GQs consist of four-stranded nucleic acid helical structures formed by the stacking of two or more guanine tetrads and stabilised by monovalent cations. GQ motifs are in fact over-represented at the ends of chromosomes, in telomeres, being involved in maintaining chromosome stability. GQ motifs are often able to inhibit telomerase action and obstruct DNA replication and repair, leading to activation of the DNA damage response pathway that results in apoptosis. The ligands reported feature a berberine G-quadruplex stabiliser scaffold connected to a moiety inhibiting hCAs IX and XII.

Crystals suitable for X-ray diffraction analysis were obtained for the human telomeric DNA sequence Tel23 in complex with the derivative S-3,2 (29). The monomolecular DNA GQ is arranged in columns growing along the c-axis and assumes the expected all-parallel conformation. In each column, symmetry-related GQ units are in stacking contact through their 5′-end G-tetrads, while the 3′-end G-tetrads constitute the binding sites. The dimers are stabilised by an additional potassium ion located between the 5′-end G-tetrads, an arrangement previously reported by several authors. Contiguous 3′-ends G-tetrads lie about 10 Å apart from one another defining a cavity big enough to host two symmetry-related ligand molecules. Each one is in contact with a 3′-end G-tetrad, and it is found to be disordered and spread over two positions, as shown in Figure 5(A,B). In both orientations the berberine core is almost planar and points the ethylenic chain towards the centre of the G-tetrad. Instead, in the propeller folding this interaction is lacking, but the three-carbon spacer connecting the oxygen and the triazole nitrogen of S-3,2 (29) has the right length to place the triazole and the benzenesulfonamide rings at stacking distance over the guanines. In the Y structure the berberine quinoline and benzo groups are at stacking distance from G22 and G16 (interplanar distances about 3.4 Å and 3.5 Å, respectively), while the triazole and the benzenesulfonamide rings are placed over the guanines G4 (3.6 Å) and G10 (3.7 Å). In the Z structure, the orientation of the molecule is flipped with respect to the Y orientation, and the G4 (interplanar distance 3.3 Å, quinoline groups’ centroids distance 3.6 Å), G10 (interplanar distance 3.3 Å, benzene groups’ centroids distance 3.9 Å) G22 (triazole ring – interplanar distance 3.4 Å) and G16 residues (benzenesulfonamide ring – interplanar distance 3.4 Å) are the most interacting.

> AGGGTTAGGGTTAGGGTTAGGGT4-CARBAMOYL-1-BETA-D-RIBOFURANOSYL-IMIDAZOLIUM-5-OLATE-5'-PHOSPHATE 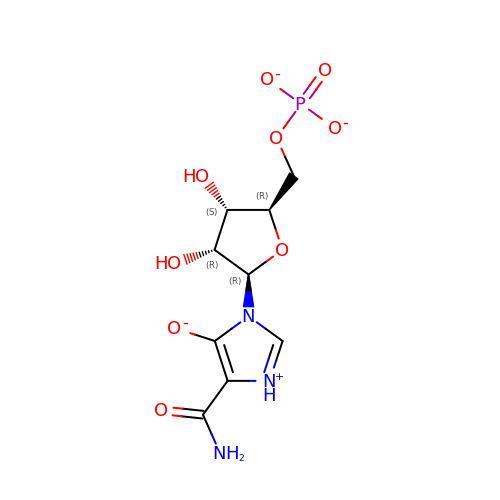| C9 H12 N3 O9 P | KTKAFSMJDTUUAN-UUOKFMHZSA-L RITONAVIR | C37 H48 N6 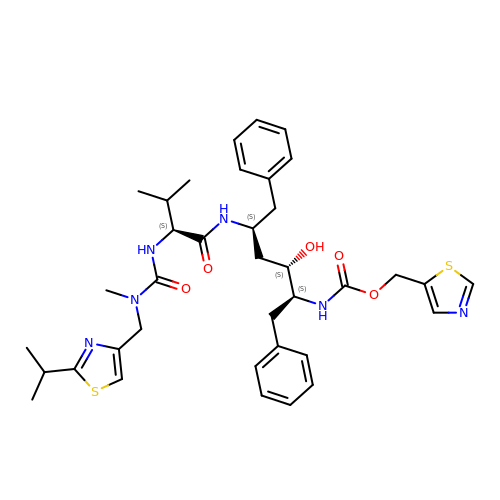O5 S2 | NCDNCNXCDXHOMX-XGKFQTDJSA-N> HHHHHHMIVL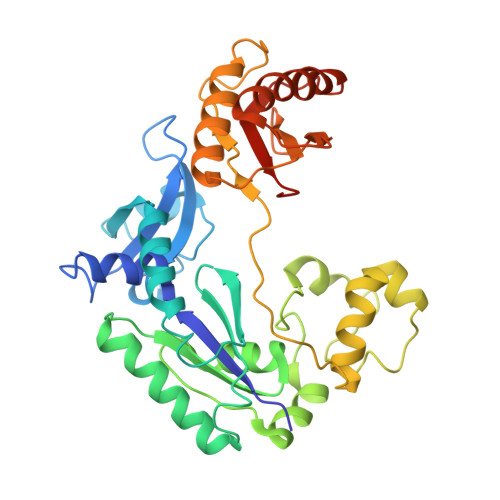FVDFDYFYAQVEEVLNPSLKGKPVVVCVFSGRFEDSGAVATANYEARKFGVKAGIPIVEAKKILPNAVYLPMRKEVYQQVSSRIMNLLREYSEKIEIASIDEAYLDISDKVRDYREAYNLGLEIKNKILEKEKITVTVGISKNKVFAKIAADMAKPNGIKVIDDEEVKRLIRELDIADVPGIGNITAEKLKKLGINKLVDTLSIEFDKLKGMIGEAKAKYLISLARDEYNEPIRTRVRKSIGRIVTMKRNSRNLEEIKPYLFRAIEESYYKLDKRIPKAIHVVAVTEDLDIVSRGRTFPHGISKETAYSESVKLLQKILEEDERKIRRIGVRFSKFIEAIGLDKFFDT>[2x]ADSDVPNDILEEQLYNSVVVADYDSAVEKSKHLYEEKKSEVITNVVNKLIRNNKMNCMEYAYQLWLQGSKDIVRDCFPVEFRLIFAENAIKLMYKRDGLALTLSNDVQGDDGRPAYGDGKDKTSPRVSWKLIALWENNKVYFKILNTERNQYLVLGVGTNWNGDHMAFGVNSVDSFRAQWYLQPAKYDNDVLFYIYNREYSKALTLSRTVEPSGHRMAWGYNGRVIGSPEHYAWGIKAF

The study reports two crystal structures of Bmlp3, a protein belonging to the 30-kDa lipoprotein family found in silkworm hemolymph. Members of the 30-kDa lipoprotein family are the most abundant protein fraction in the hemolymph of silkworm fifth instar larvae. The Bmlp3 molecule consists of a helical N-terminal domain (NTD, residues 1–87) and a β-trefoil C-terminal domain (CTD, residues 88–239). The NTD consists of six helices forming a right-handed superhelix and is classified as a VHS domain.

The crystal structure of the second crystal form (Bmlp3-c2) was solved using a model (Bmlp3-p21) with the correct amino acid sequence. There are two protein molecules in the asymmetric unit of the Bmlp3-c2 crystal. The Bmlp3-c2 model contains residues 5–239 in each chain. The dimer present in the Bmlp3-c2 structure is formed through interactions between the CTD domains in a tail-to-tail arrangement. The results of PISA analysis of the Bmlp3-c2 structure suggest that the dimer present in the asymmetric unit could be also stable in solution. The interaction interface between the CTDs of protein molecules A and B is formed mainly by amino acid residues in loops β2–β3 and β6–β7. In molecule A this loop is shifted by about 5 Å compared to the same loop in Bmlp3–p21, whereas in molecule B this shift is about twice as large and the loop is bent. Such an arrangement of loop 106–116 in both protein molecules stabilizes the dimer. The central part of the dimerization interface is occupied by an iodide anion from the crystallization solution. The iodide anion forms hydrogen bonds with three water molecules, with I…O distances ranging from 3.2 to 3.7 Å, and with two nitrogen atoms of the protein backbone (Gly158A/B) with the N…I distances of 3.7 and 3.9 Å.2-(acetylamino)-2-deoxy-1-O-[(S)-hydroxy{[(S)-hydroxy{[(2Z,6Z,10Z,14Z,18Z,22Z,26Z)-3,7,11,15,19,23,27,31-octamethyldotriaconta-2,6,10,14,18,22,26,30-octaen-1-yl]oxy}phosphoryl]oxy}phosphoryl]-alpha-D-glucopyranose | C48 H81 N O12 P2 | 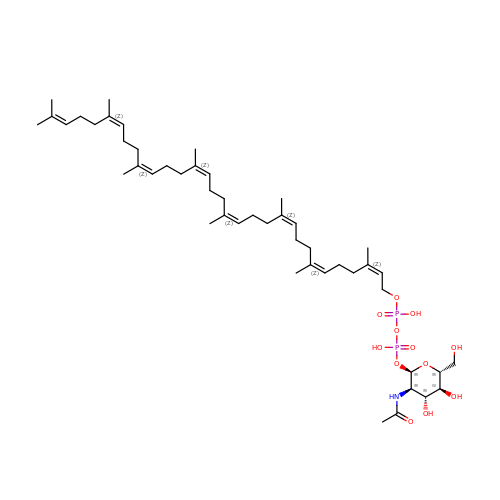UHEQUFGFBDQLSB-MUZKLJMZSA-N>GSFSDETLDKVPKSEGYCSRILRAQGTRREGYTEFSLRVEGDPDFYKPGTSYRVTLSAAPPSYFRGFTLIALRENREGDKEEDHAGTFQIIDEEETQFMSNCPVAVTESTPRRRTRIQVFWIAPPAG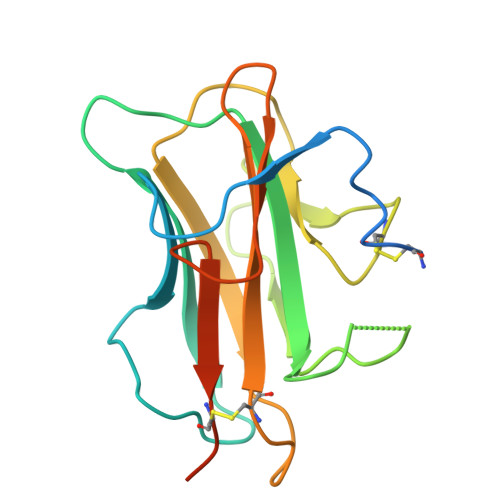TGCVILKASIVQKRIIYFQDEGSLTKKLCEQDSTFDGVTDKPILD[4x]> ETVSTQELYSIPEDQEPEDQEPEEPTPAPWARLWALQDGFANLECVNDNYWFGRDKSCEYCFDEPLLKRTDKYRTYSKKHFRIFREVGPKNSYIAYIEDHSGNGTFVNTELVGKGKRRPLNNNSEIALSLSRNK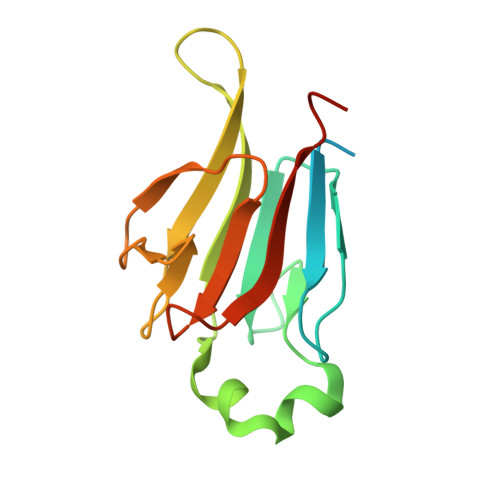VFVFFDLTVDDQSVY>[2x]MEFLNSIPWEEVVPGQFTANPGFQVTDYFEIVRQPADGNCFYHSIAELFVPNKNDFSFRLVKQHLELAARRFFEEESEAKGLGLSLEKYLEVAMCDNEWGGSLEASMLAKHLDITIVIWVIEGPSRVAAAVKFGPGDVAGAINLLHTGYNHFDALRLLVDDSQVSRQPRSGSHHHHHH;>[2x]MGGDLKVKMLGGEEILVPLRDSMMVSELKQFIAQKINVPAFQQRLAHLDSREVLQEGVPLVHQGLKAGSTILLMVQNSSATLNILVRNDKGRSSSYEVQLTQTVAVLKQQVCQRERVQADQFWLSFEGKPMDDEHPLGEYGLTTGCTVFMNLRLRG

Beyond the RNA-dependent RNA polymerase (RdRp), the L protein contains a viral homologue of the ovarian tumor domain protease (OTU) at the N-terminus. This OTU reverses posttranslational modifications by ubiquitin (Ub) and interferon (IFN) stimulated gene product 15 (ISG15). Sheep ISG15 was derivatized into a suicide inhibitor with propargylamine and incubated with KUPEV and GANV OTUs to form covalent complexes that could be used for X-ray crystallography. This yielded an atomic resolution structure of KUPEV OTU bound to the C-terminal domain of sheep ISG15 (C-sheep ISG15) solved to 2.06 Å and a low-resolution structure of GANV OTU bound to full length sheep ISG15 to 3.15 Å.

GANV and KUPEV OTUs interact with sheep ISG15 in a highly similar manner, including how GANV OTU accommodates sheep ISG15 D89 outside of the selectivity pocket. Given that both OTUs of GANV and KUPEV exhibit robust deISGylation activity towards sheep ISG15, this highlights that accommodation of D89 in the selectivity pocket is not necessary for robust OTU deISGylase activity. The most noticeable difference in the interface of the OTUs from KUPEV and GANV with sheep ISG15 is located at position 122. For GANV OTU, this position is occupied by a glutamate that is in proximity to interact with sheep ISG15’s K90. In the KUPEV OTU residue 122 is an asparagine residue, while CCHFV is unique among OTUs with an alanine at this position. These residues would not have the same potential to interact with ISG15 or Ub substrates as E122 in GANV OTU, suggesting this may partially account for the observed enhanced activity of GANV OTU towards Ub and human ISG15-7-amido-4-methylcoumarin (AMC) substrates. As anticipated, the GANV OTU E122N mutant reduced activity for human ISG15-AMC almost 10-fold, while KUPEV OTU N122E boosted activity more than 6-fold relative to WT. Despite being a variant of the same virus, GANV possesses enhanced activity towards human, camel, pig, and mouse proISG15. In GANV and CCHFV residue 80 is a lysine and arginine, respectively, which are both flexible and capable of forming an electrostatic interaction. For GANV OTU, the K80I mutant reduces human ISG15-AMC activity by half but does not affect Ub-AMC, while the helix mutant reduces both by approximately half.>MWHTHSEREKRVSNAVEF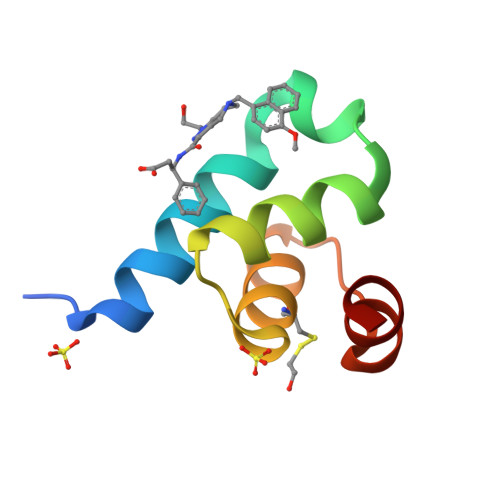LLDSRVRRTPTSSKVHFLKSKGLSAEEICEAFTKVGQPKTLNEIKRILS[4x]>EAQRQFARVKLPARIRYIGANREGVDARLLDLSAGGFAFTASGAPIQPGDLYKGKMLFQVDSISFSLEVEFQVRSVDPASRRVGCEFQNLKPREVAALRYLIT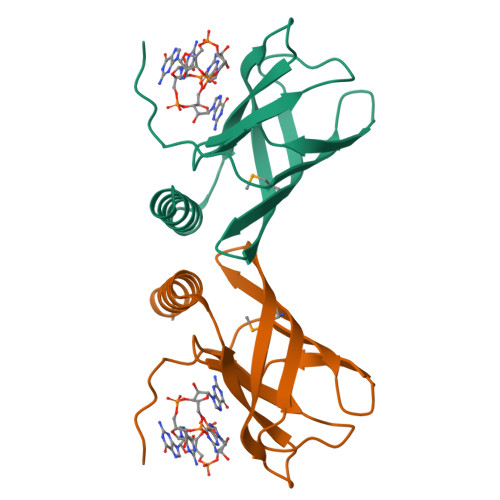SYLAGERQA[3x]>GIDPFTFENATSDAINQDMMLYIERIAKIIQKLPKRVHINVRGFTDDTPLVKTRFKSHYELAANRAYRVMKVLIQYGVNPNQLSFSSYGSTNPIAPNDSLENRMKN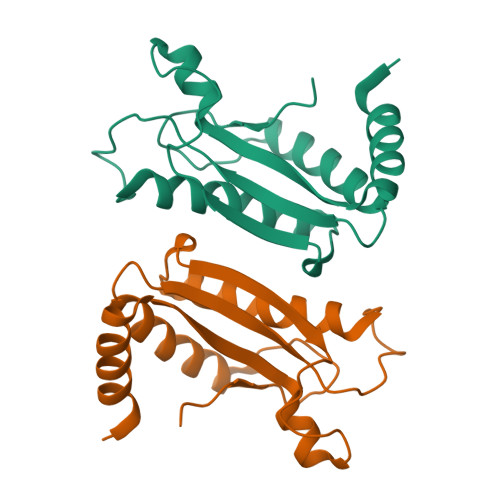NRVEIFFSTDANDLSKIHSILDNEFNPHKQQE[12x]>[2x]ACGLVASNLNLKPGECLKVRGELAPDAKSFV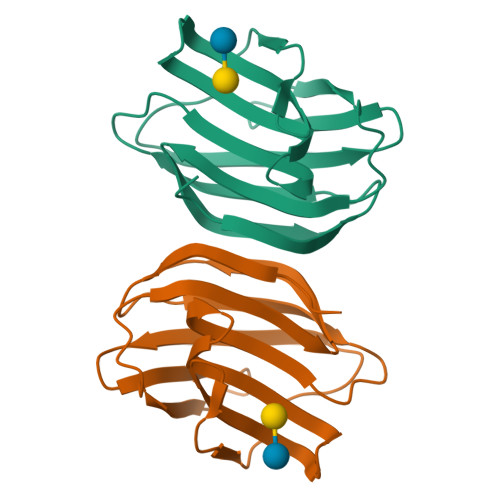LNLGKDSNNLCLHFNPRFNAHGDANTIVCNSKDDGTWGTEQRETAFPFQPGSITEVCITFDQADLTIKLPDGHEFKFPNRLNMEAINYMAADGDFKVKCVAFE> SSYSGPIVVDPVTRIEGHLRIEVEVENGKVKNAYSSSTLFRGLEIILKGRDPRDAQHFTQRTCGVCTYTHALASTRCVDNAVGVHIPKNATYIRNLVLGAQYLHDHIVHFYHLHALDFVDVTAALKADPAKAAKVASSISPRKTTAADLKAVQDKLKTFVETGQLGPFTNAYFLGGHPAYYLDPETNLIATAHYLEALRLQVKAARAMAVFGAKNPHTQFTVVGGVTCYDALTPQRIAEFEALWKETKAFVDEVYIPDLLVVAAAYKDWTQYGGTDNFITFGEFPKDEYDLNSRFFKPGVVFKRDFKNIKPFDKMQIEEHVRHSWYEGAEARHPWKGQTQPKYTDLHGDDRYSWMKAPRYMGEPMETGPLAQVLIAYSQGHPKVKAVTDAVLAKLGVGPEALFSTLGRT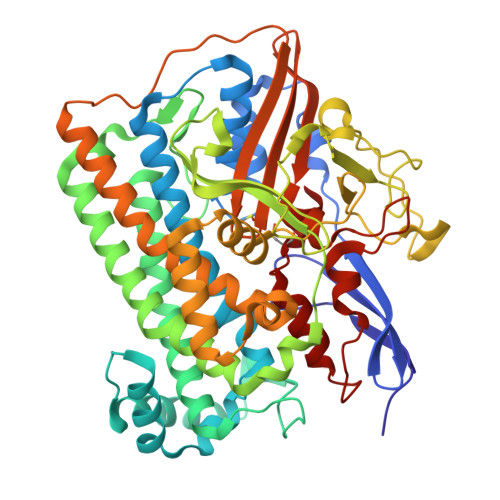AARGIETAVIAEYVGVMLQEYKDNIAKGDNVICAPWEMPKQAEGVGFVNAPRGGLSHWIRIEDGKIGNFQLVVPSTWTLGPRCDKNKLSPVEASLIGTPVADAKRPVEILRTVHSFDPCIACGVH>[4x]MTKIALIGSGQIGAIVGELCLLENLGDLILYDVVPGIPQGKALDLKHFSTILGVNRNILGTNQIEDIKDADIIVITAGVQRKEGMTREDLIGVNGKIMKSVAESVKLHCSKAFVICVSNPLDIMVNVFHKFSNLPHEKICGMAGILDTSRYCSLIADKLKVSAEDVNAVILGGHGDLMVPLQRYTSVNGVPLSEFVKKNMISQNEIQEIIQKTRNMGAEIIKLAKASAAFAPAAAITKMIKSYLYNENNLFTCAVYLNGHYNCSNLFVGSTAKINNKGAHPVEFPLTKEEQDLYTESIASVQSNTQKAFDLIKAAALEHHHHHH

Malate dehydrogenases are a group of multimeric enzymes, typically self-organized as dimers or tetramers, that reversibly catalyze the oxidation of malate to oxaloacetate using the reduction of NAD+ to NADH as a cofactor. Malate dehydrogenases (MDHs) sustain tumor growth and carbon metabolism by pathogens including Plasmodium falciparum. However, clinical success of MDH inhibitors is absent, as current small molecule approaches targeting the active site are unselective. The presence of an allosteric binding site at oligomeric interface allows the development of more specific inhibitors.

In addition, the atomic coordinates of the loop R75-I87 located between helices α3 and β4 sheet of the catalytic site of chains A–C were omitted due to a lack of electron density, caused by an increase in local structural flexibility. Similarly, disordered active site loops were observed in the NADH bound form and no electron density is observed for residues Q80–L90. Eighteen identical residues (G8, G10, L30, D32, G40, D71, G84, D89, L90, N94, P120, L146, S227, and A233 with D147, R150, R87, and N119) cluster at the N-terminal cofactor binding domain (Rossmann-fold). Five of these (H174, R150, R87, R81, and D147) are involved in the catalytic mechanism where the three arginines interact with the carboxylates groups of the substrate (malate or oxaloacetate) through ionic contacts. Overall, the three independent oligomeric interfaces of PfMDH possess a buried solvent accessible surface area of 3481 Å2. In contrast, the AB and AC interfaces represent the key contact surface for the oligomerization (1811 and 1309 Å2, respectively) and are essential for the biological activity in vitro.Poliovirus (PV) belongs to the Enterovirus genus of the Picornaviridae family. The PV genome, approximately 7.5 kb in length, is a single-stranded, positive-sense RNA enclosed within a capsid protein shell. The P1 is further cleaved by a viral protease to produce the capsid subunit proteins VP0, VP1, and VP3. In this study, we investigate the production, antigenicity, thermostability, immunogenicity, and structures of VLPs derived from PV serotype 2 (PV2) wildtype strain and thermally stabilized mutant (wtVLP and sVLP, respectively).

Our cryo-EM analysis revealed that the PV2 sVLP closely resembles the native mature virion in the capsid region, whereas the PV2 wtVLP adopts an expanded conformation similar to the EC or 135S particle. However, the wtVLP appears to be in an expanded state compared to the sVLP, as evidenced by the radius of the wtVLP being 170 Å and that of the sVLP being 163 Å. Structural comparison revealed that the two-fold axis channel, formed by VP2 and VP3, is markedly opened in the wtVLP, whereas it is closed in the sVLP. Detailed structural analysis shows that in the wtVLP, the pocket factor binding site is preoccupied by the side chains of Y159, F237, and N235, and the hydrophobic pocket collapsed, with its volume reducing from 914 Å3 to 577 Å3 (measured by ProteinsPlus). As a result, the wtVLP VP1 “pocket” can no longer accommodate lipids. The structural comparison showed that the wtVLP is highly similar to the PV1 135S-like particles, and the sVLP structure aligns well with the native PV2 model. Moreover, the B-factor of the sVLP is generally lower than that of the wtVLP. Collectively, the increase in the number of ordered parts of capsid proteins and lower B-factor suggest that the sVLP is more structurally stable than the wtVLP. The D-antigen content (reflected by the binding activity to the mAb 1050) in the wtVLP dropped drastically at 35 °C and was almost completely lost at 40 °C, whereas the sVLP exhibited significantly improved D-antigenic thermostability, maintaining >50% D-antigen content even at 45 °C. Next, we treated wtVLP and sVLP at 37 °C for different periods of time and then evaluated total antigen and D-antigen content. Despite the yeast-derived wtVLP also possessing a reasonable amount of D-antigen, it fails to trigger a neutralizing antibody response in vivo, likely due to its poor thermostability especially at 37 °C, the normal physiological temperature of mice and humans.

> GLGDLIEGVVEGVTRNALTPLTPANNLPDTQSSGPAHSKETPALTAVETGATNPLVPSDTVQTRHVIQKRTRSESTVESFFARGACVAIIEVDNDAPTKRASKLFSVWKITYKDTVQLRRKLEFFTYSRFDMEFTFVVTSNYTDANNGHALNQVYQIMYIPPGAPIPGKWNDYTWQTSSNPSVFYTYGAPPARISVPYVGIANAYSHFYDGFAKVPLAGQASTEGDSLYGAASLNDFGSLAVRVVNDHNPTKLTSKIRVYMKPKHVRVWCPRPPRAVPYYGPGVDYKDGLAPLPEKGLTTY;> SPNIEACGYSDRVMQLTLGNSTITTQEAANSVVAYGRWPEYIKDSEANPVDQPTEPDVAACRFYTLDTVTWRKESRGWWWKLPDALKDMGLFGQNMFYHYLGRAGYTVHVQCNASKFHQGALGVFAVPEMCLAGDSTTHMFTKYENANPGEKGGEFKGSFTLDTNATNPARNFCPVDYLFGSGVLAGNAFVYPHQIINLRTNNCATLVLPYVNSLSIDSMTKHNNWGIAILPLAPLDFATESSTEIPITLTIAPMCCEFNGLRNITVPRTQ;> GLPVLNTPGSNQYLTADNYQSPCAIPEFDVTPPIDIPGEVRNMMELAEIDTMIPLNLTNQRKNTMDMYRVELNDAAHSDTPILCLSLSPASDPRLAHTMLGEILNYYTHWAGSLKFTFLFCGSMMATGKLLVSYAPPGAEAPKSRKEAMLGTHVIWDIGLQSSCTMVVPWISNTTYRQTINDSFTEGGYISMFYQTRVVVPLSTPRKMDILGFVSACNDFSVRLLRDTTHISQEAMPQ> QRAKVAMSHFEPHEYIRYDLLEKNIDIVRKRLNRPLTLSEKIVYGHLDDPANQEIERGKTYLRLRPDRVAMQDATAQMAMLQFISSGLPKVAVPSTIHCDHLIEAQLGGEKDLRRAKDINQEVYNFLATAGAKYGVGFWRPGSGIIHQIILENYAYPGVLLIGTDSHTPNGGGLGGICIGVGGADAVDVMAGIPWELKCPKVIGVKLTGSLSGWTSPKDVILKVAGILTVKGGTGAIVEYHGPGVDSISCTGMATICNMGAEIGATTSVFPYNHRMKKYLSKTGRADIANLADEFKDHLVPDSGCHYDQLIEINLSELKPHINGPFTPDLAHPVAEVGSVAEKEGWPLDIRVGLIGSCTNSSYEDMGRSAAVAKQALAHGLKCKSQFTITPGSEQIRATIERDGYAQVLRDVGGIVLANACGPCIGQWDR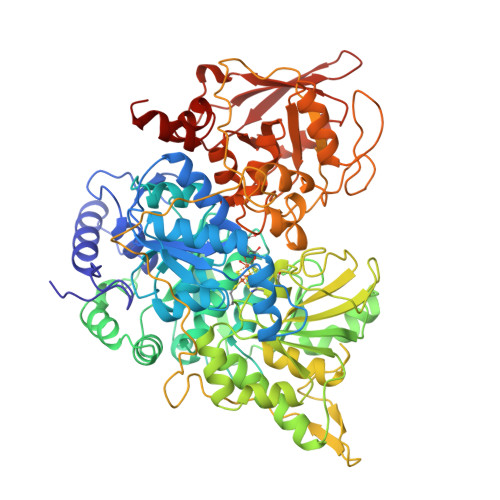KDIKKGEKNTIVTSYNRNFTGRNDANPETHAFVTSPEIVTALAIAGTLKFNPETDFLTGKDGKKFKLEAPDADELPRAEFDPGQDTYQHPPKDSSGQRVDVSPTSQRLQLLEPFDKWDGKDLEDLQILIKVKGKCTTDHISAAGPWLKFRGHLDNISNNLLIGAINSENRKANSVRNAVTQEFGPVPDTARYYKQHGIRWVVIGDENYGEGSSREHSALEPRFLGGRAIITKSFARIHETNLKKQGLLPLTFADPADYNKIHPVDKLTIQGLKDFAPGKPLTCIIKHPNGTQETILLNHTFNETQIEWFRAGSALNRMKELQQK>GSEERRYKRCGQDEERVRRECKERGERQNCQYQIRKEGNCYVCEI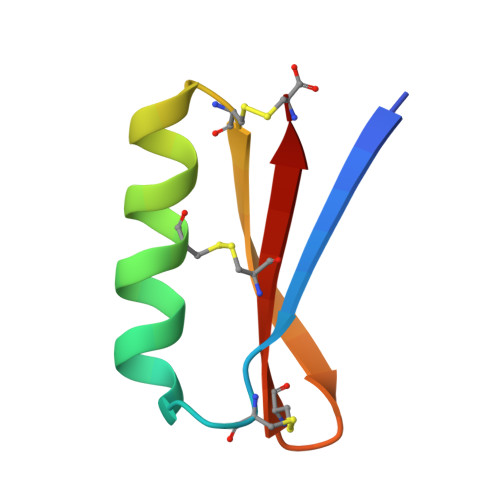RC[3x]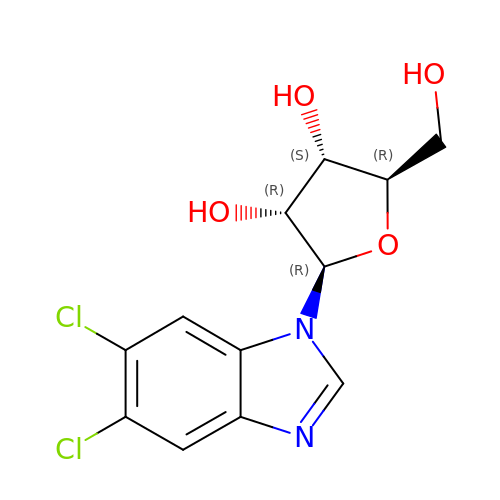5,6-dichloro-1-beta-D-ribofuranosyl-1H-benzimidazole | C12 H12 Cl2 N2 O4 | XHSQDZXAVJRBMX-DDHJBXDOSA-N>MCTGLRFTDEQGNLYFGRNLDVGQDYGEGVIITPRHYPLPYKFLD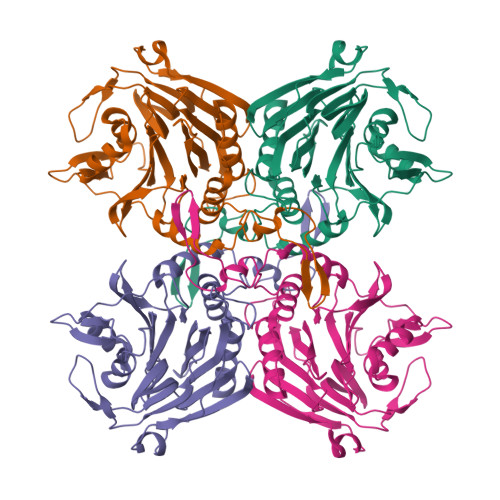NTTTKKAVIGMGIVVDGYPSYFDCYNEDGLGIAGLNFPHFAKFSDGPIDGKINLASYEIMLWVTQNFTHVSEVKEALKNVNLVNEAINSSFAVAPLHWIISDSDEAIIVEVSKQYGMKVFEDKLGVLTNSPDFNWHLTNLGNYTGLNPHDATAQSWNGQKVAPWGVGTGSLGLPGDSIPADRFVKAAYLNANYPAAKGEKANVAKFFNILKSVAMIKGSVVNVQGKDEYTVYTACYSSGSKTYYCNFEDDFELKTYKLDDKTMNSTSLITYHHHHHH[4x]>MSYDVVIPAAGQGKRMKAGRNKLFIELKGDPVIIHTLRVFDSHRQCDKIILVINEQEREHFQQLLSDYPFQTSIELVAGGDERQHSVYKGLKAVKQEKIVLVHDGARPFIKHEQIDELIAEAEQTGAAILAVPVKDTIKRVQDLQVSETIERSSLWAVQTPQ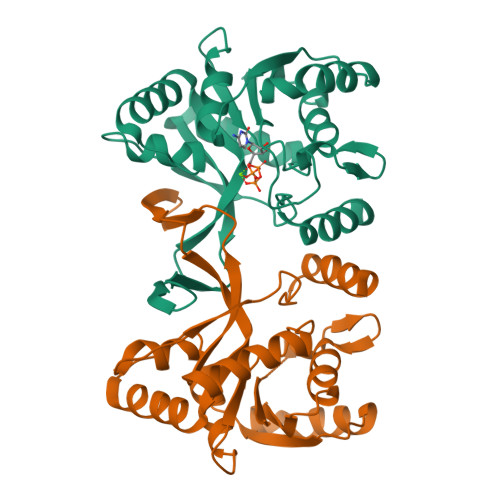AFRLSLLMKAHAEAERKGFLGTDDASLVEQMEGGSVRVVEGSYTNIKLTTPDDLTSAEAIMESESGNKHV[2x]>GAPATVAEQGEDITSKKD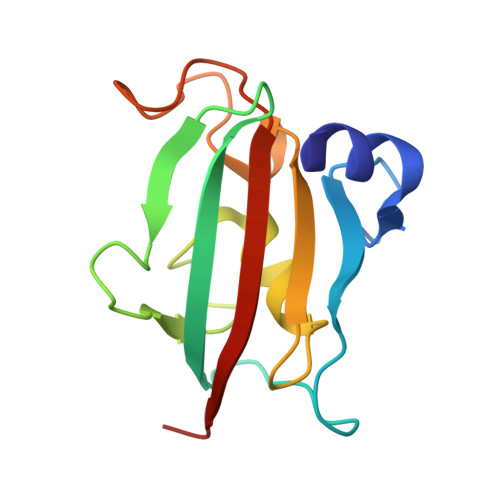RGVLKIVKRVGNGEETPMIGDKVYVHYKGKLSNGKKFDSSHDRNEPFVFSLGKGQVIKAWDIGVATMKKGEICHLLCKPEYAYGSAGSLPKIPSNATLFFEIELLDFKGE[2x]>MATLSLTVNSGDPPLGALLAVEHVKDDVSISVEEGKENILHVSENVIFTDVNSILRYLARVATTAGLYGSNLMEHTEIDHWLEFSATKLSSCDSFTSTINELNHCLSLRTYLVGNSLSLADLCVWATLKGNAAWQEQLKQKKAPVHVKRWFGFLEAQQAFQSVGTKWDVSTTKAR[4x];>MTNIIQADEPTTLTTNALDLNSVLGKDYGALKDIVINANPASPPLSLLVLHRLLCEHFRVLSTVHTHSSVKSVPENLLKCFGEQNKKQPRQDYQLGFTLIWKNVPKTQMKFSIQTMCPIEGEGNIARFLFSLFGQKHNAVNATLIDSWVDIAIFQLKEGSSKEKAAVFRSMNSALGKSPWLAGNELTVADVVLWSVLQQIGGCSVTVPANVQRWMRSCENLAPFNTALKLLKLEHHHHHH[4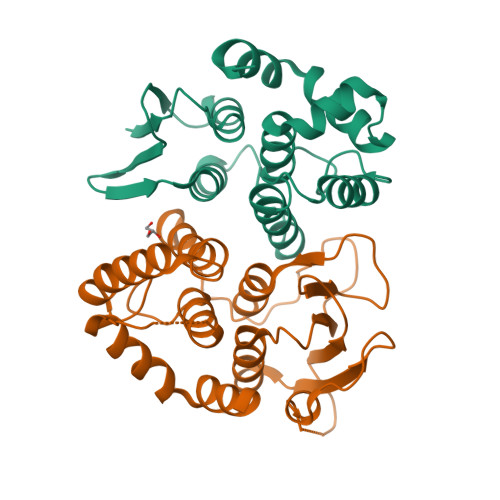x]>[4x]TETTSFSITKFGPDQQNLIFQGDGYTTKERLTLTKAVRNTVGRALYSSPIHIWDSKTGNVANFVTSFTFVIDAPNSYNVADGFTFFIAPVDTKPQTGGGYLGVFNSKDYDKTSQTVAVEFDTFYNTAWDPSNGDRHIGI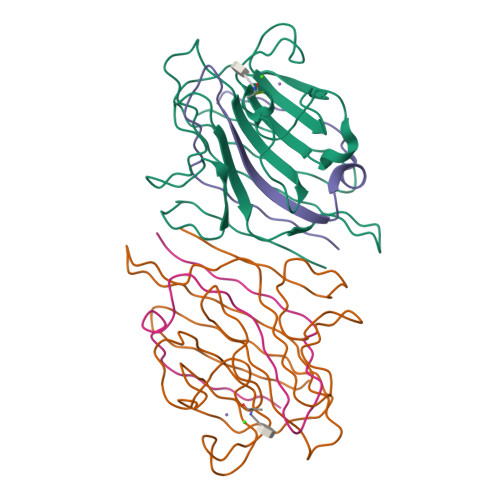DVNSIKSINTKSWALQNGKEANVVIAFNAATNVLTVSLTYPN;>ETSYTLNEVVPLKEFVPEWVRIGFSATTGAEFAAHEVLSWYFHSELAGTSSS[4x]>[4x]MATRSPGVVISDDEPGY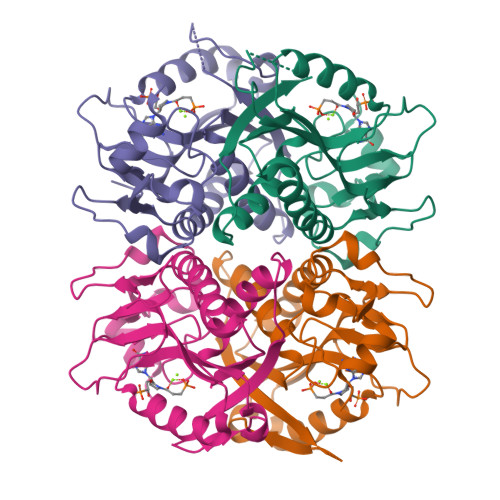DLDLFAIPNHYAEDLERVFIPHGLIMDRTERLARDVMKEMGGHHIVALCVLKGGYKFFADLLDYIKALNRNSDRSIPMTVDFIRLKSYCNDQSTGDIKVIGGDDLSTLTGKNVLIVEDIIDTGKTMQTLLSLVRQYNPKMVKVASLLVKRTPRSVGYKPDFVGFEIPDKFVVGYALDYNEYFRDLNHVAVISETGKAKYKA>MAHHHHHHMKNVLSIQSHVIYGHAGNS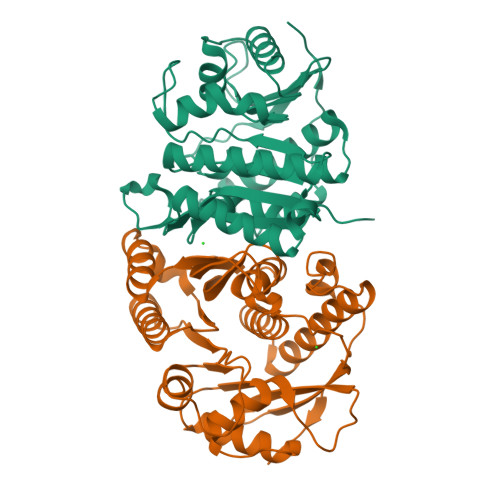AAVFPMQRLGVNVWPLNTVQLSNHMQYGHWAGSAIDAAKMEQLVDGIAAIGALKRCDAVLSGFAGSPAQARATVEIVRAVKAMNPNAWYFCDPAMGQTGGIRPEPGVEEFIVNEMPALADGMSPNHTELQKLAGRRIETVAEAVDACRTLIARGPKIILVKHLHDRNSPADRFNMLAVTETEAWIGQRPLYAFPRHPVGVGDLTSAIFVARRLRGDSVRAAFEHTLAAVHAVVKATYDARRYELELIAAQDEIARPSEWFGAWVTDV[2x]Clathrin-mediated endocytosis is essential for protein retrieval during neurotransmission and receptor recycling. Accumulation of the adapter proteins at the plasma membrane initiates the endocytic event and contributes to membrane bending. Complex formation has been observed between the ENTH domain of epsin and the ANTH domain of Sla2, the yeast homolog of human huntingtin interacting protein 1 related (Hip1R). Epsin and the phospholipid PIP2 are essential for clathrin-mediated endocytosis, and we show how assemblies are formed between the ENTH domain of epsin and the ANTH domain of Sla2 in fungi.

To understand why the ANTH domain of Sla2/Hip1R is specifically suited to bind the ENTH domain of epsins through the lipid interface, we determined the crystal structure of the ANTH domain of homologous Sla2 from C. thermophilum to 1.8 Å resolution. The overall ANTH fold consists of helices α1–α11 and is conserved between CALM and Sla2/Hip1R subfamilies. Through insertion of a conserved Tyr 252 and a hydrophobic residue, an extra α helix (α12) uniquely occurs in Sla2 ANTH domains, providing rigidity. A loop connecting helices α8 and α9 has a five-residue extension in Sla2, although with non-conserved sequence. Based on the low-resolution electron microscopy tomogram of the Ent1 ENTH/ANTH Sla2 complex from S. cerevisiae, these insertions point at the epsin interface. Moreover, deleting the Sla2/Hip1R-specific α12 helix impaired the function of the Sla2 ANTH domain similarly to mutating Arg 29, which is essential for the ENTH/ANTH complex formation. Based on the C. thermophilum Sla2 ANTH crystal structure, ANTH domains of the Sla2/Hip1R subfamily do not contain an N-terminal α helix. A crystal structure of the Sla2 ANTH domain from C. thermophilum reveals that Hip1R-related ANTH domains have two evolutionarily conserved insertions that contribute to the epsin/Hip1R interface to enable PIP2-dependent ENTH/ANTHSla2 complex formation. Especially the insertion of an α helix around Tyr 252 provides surface complementarity in the ENTH/ANTHSla2-binding interface, compared to the structures of the ANTH domains of AP180/CALM proteins. In addition, residue Arg 37 can toggle its side chain between the canonical PIP2-binding site of ANTH domains, and the ENTH/ANTHSla2 interface.

>SLDHAKAEAELAINIKKATSPEETAPKRKHVRSCIVYTWDHKSSLSFWAGLKVQPILADEVQTFKALITIHKVLQEGHPVTLREAMANRGWIDSLSRGMMGEGVRGYGPLIREYVHFLLAKLSFHKQHPEFNGTFEYEEYISLKAIHDPNEGYETITDLMTLQDKIDQFQKLIFSHFRHIGNNECRISALVPLVAESYGIYKFITSMLRAMHSSTGDNEALEPLRQRYDAQHYRLVKFYYECSNLRYLTSLITIPKL[2x]> GKFKLVFLGEQSVGKTSLITRFMYDSFDNTYQATIGIDFLSKTMYLEDRTVRLQLWDTAGQERFRSLIPSYIRDSTVAVVVYDITNLNSFQ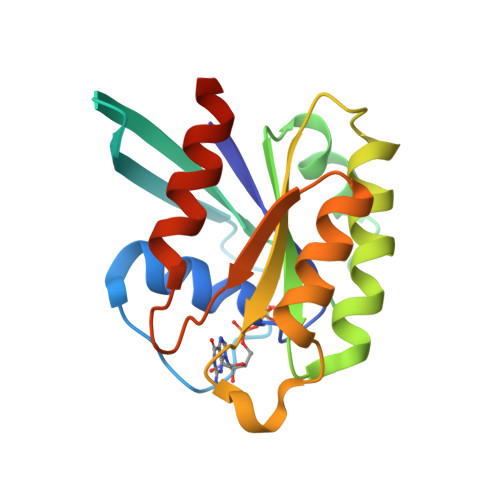QTSKWIDDVRTERGSDVIIMLVGNKTDLADKRQITIEEGEQRAKELSVMFIETSAKTGYNVKQLFRRVASALLEHHHHHH> MFPAAPSPRTPGTGSRRGPLAGLGPGSTPRTASRKGLPLGSAVSSPVLFSPVGRRSSLSSRGTPTRMFPHHSITESVNYDVKTFGSSLPVKVMEALTLAEVDDQLTINIDEGGWACLVCKEKLIIWKIALSPITKLSVCKELQLPPSDFHWSADLVALSYSSPSGEAHSTQAVAVMVATREGSIRYWPSLAGEDTYTEAFVDSGGDKTYSFLTAVQGGSFILSSSGSQLIRLIPESSGKIHQHILPQGQGMLSGIGRKVSSLFGILSPSSDLTLSSVLWDRERSSFYSLTSSNISKWELDDSSEKHAYSWDINRALKENITDAIWGSESNYEAIKEGVNIRYLDLKQNCDGLVILAAAWHSADNPCLIYYSLITIEDNGCQMSDAVTVEVTQYNPPFQSEDLILCQLTVPNFSNQTAYLYNESAVYVCSTGTGKFSLPQEKIVFNAQGDSVLGAGACGGVPIIFSRNSGLVSITSRENVSILAEDLEGSLASSVAGPNSESMIFETTTKNETIAQEDKIKLLKAAFLQYCRKDLGHAQMVVDELFSSHSDLDSDSELDRAVTQISVDLMDDYPASDPRWAESVPEEAPGFSNTSLIILHQLEDKMKAHSFLMDFIHQVGLFGRLGSFPVRGTPMATRLLLCEHAEKLSAAIVLKNHHSRLSDLVNTAILIALNKREYEIPSNLTPADVFFREVSQVDTICECLLEHEEQVLRDAPMDSIEWAEVVINVNNILKDMLQAASHYRQNRNSLYRREESLEKEPEYVPWTATSGPGGIRTVIIRQHEIVLKVAYPQADSNLRNIVTEQLVALIDCFLDGYVSQLKSVDKSSNRERYDNLEMEYLQK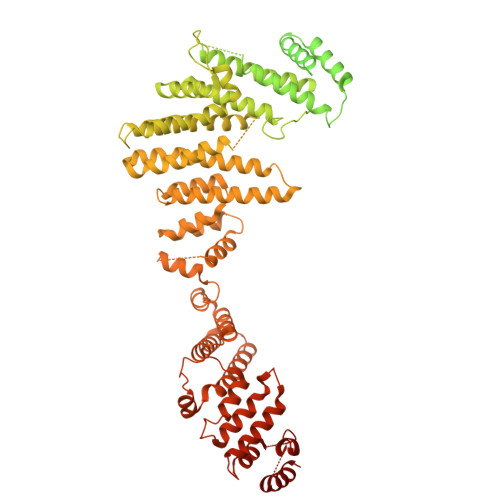RSDLLSPLLSLGQYLWAASLAEKYCDFDILVQMCEQTDNQSRLQRYMTQFADQNFSDFLFRWYLEKGKRGKLLSQPISQHGQLANFLQAHEHLSWLHEINSQELEKAHATLLGLANMETRYFAKKKTLLGLSKLAALASDFSEDMLQEKIEEMAEQERFLLHQETLPEQLLAEKQLNLSAMPVLTAPQLIGLYICEENRRANEYDFKKALDLLEYIDEEEDININDLKLEILCKALQRDNWSSSDGKDDPIEVSKDSIFVKILQKLLKDGIQLSEYLPEVKDLLQADQLGSLKSNPYFEFVLKANYEYYVQGQI>GHMNLCYIDGKFLPLEEAKLPVTDLIIQRGVGVFETISTHSRRPLMLTPHLKRLEGSATASSIVMPATLDEMARIIREGIKKMGCETMVRPYITGGDSFGKDHLFSSSRYFVIFEEIRKPDPILYEKGVALHPINAERYLPSTKSINYMLSFTGQRDSKGAYEILYCPEGEIVEGSHSTFFLIKNGHLITAPTSRALSGTTRQIVLELARRGNIQVEERCPLLTELPEAEEAFITGTVKE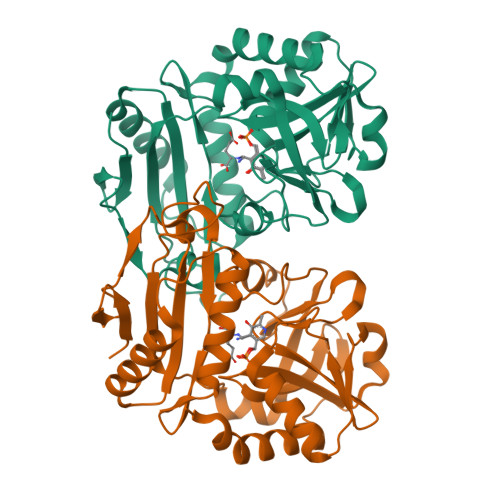LLPVVRIGDQIIGNGVPGKLTKHLHQVYLSSIVEWLE[2x]> MAHHHHHHADLPIMHDSDRYELVKDIGSGNFGVARLMRDKQSNELVAVK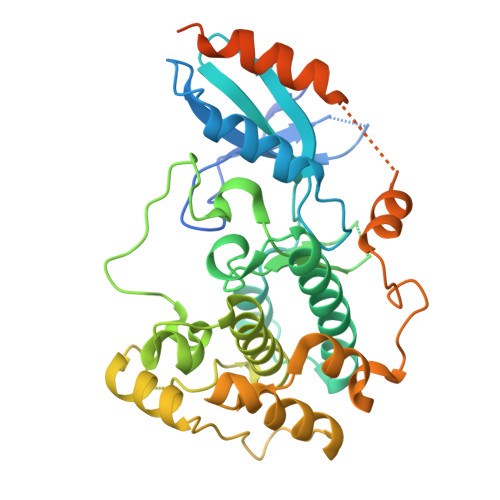YIERGEKIDENVKREIINHRSLRHPNIVRFKEVILTPTHLAIVMEYASGGELFERICNAGRFSEDEARFFFQQLISGVSYCHAMQVCHRDLKLENTLLDGSPAPRLKICDFGYSKSSVLHSQPKSTVGTPAYIAPEVLLKKEYDGKVADVWSCGVTLYVMLVGAYPFEDPEEPKNFRKTIHRILNVQYAIPDYVHISPECRHLISRIFVADPAKRISIPEIRNHEWFLKNLPADLMNDNTMTTQFAASDQPGQSIEEIMQIIAEATVPPAGTQNLNHYLTGSLDIDDDMEEDLESDLDDLDIDSSGEIVYAM> QPIFLNVLEAIEPGVVCAGHDNNQPDSFAALLSSLNELGERQLVHVVKWAKALPGFRNLHVDDQMAVIQYSLMGLMVFAMGWRSFTNVNSAMLYFAPDLVFNEYRMHK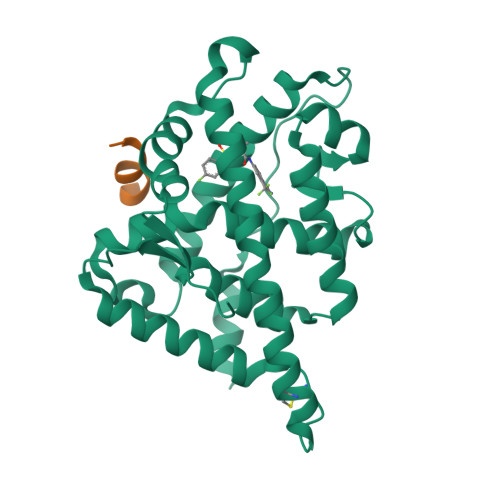SRMYSQCVRMRHLSQEFGWLQITPQEFLCMKALLLFSIIPVDGLKNQKFFDELRMNYIKELDRIIACKRKNPTSCSRRFYQLTKLLDSVQPIARELHQFTFDLLIKSHMVSVDFPEMMAEIISVQVPKILSGKVKPIYFHTQ;> RGAFQNLFQSV> MRGSHHHHHHGSIQKTTIAADSSSKPRGINYDTGIPFNVLIVDDSVFTVKQLTQIFTSEGFNIIDTAADGEEAVIKYKNHYPNIDIVTLDITMPKMDGITCLSNIMEFDKNARVIMISALGKEQLVKDCLIKGAKTFIVKPLDRAKVLQRVMSVFVK;> MRGSHHHHHHGSRIDYIEPF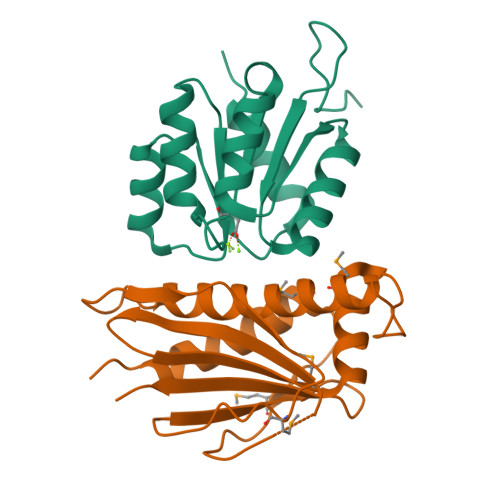LDAASSVLRDMLLVENIEMGKPGLKSINQKIKGVSVIVGLAGSVEGSIIIDMDIETALFVASKLNFEEYDDFDDEETKEMVAATLTEVGNIIAGNFVTTLHAKGFVFDITPPAFIYGENMKISNKGSEALIVPFSLPDGKIIEVNIAIRERV> SLLTCGGCQQNIGDRYFLKAIDQYWHEDCLSCDLCGCRLGEVGRRLYYK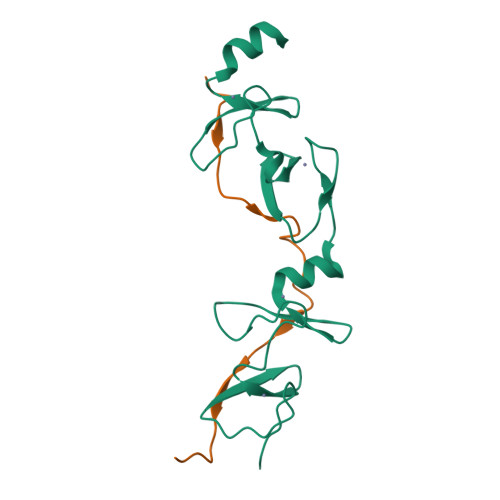LGRKLCRRDYLRLFGQDGLCASCDKRIRAYEMTMRVKDKVYHLECFKCAACQKHFCVGDRYLLINSDIVCEQDIYEWTKING;> VPDVMVVGEPTLMGGEFGDEDERLITRLENTQFDA>MKKAWCWASYLEEEKAVAVPAKLFKEHQSFPYNKNGFKVGMKLEGVDPEHQSVYCVLTVAEVCGYRIKLHFDGYSDCYDFWVNADALDIHPVGWCEK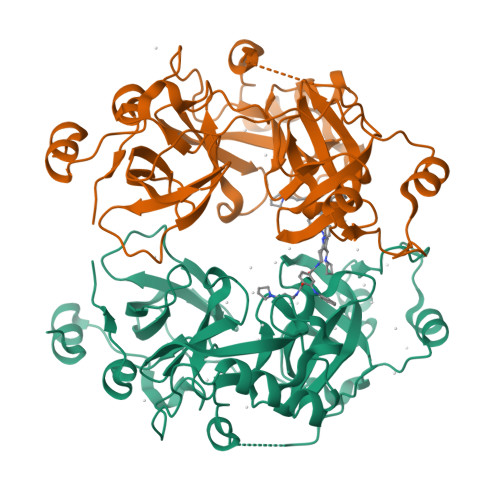TGHKLHPPKGYKEEEFNWQTYLKTCKAQAAPKSLFENQNITVIPSGFRVGMKLEAVDKKNPSFICVATVTDMVDNRFLVHFDNWDESYDYWCEASSPHIHPVGWCKEHRRTLITPPGYPNVKHFSWDKYLEETNSLPAPARAFKVKPPHGFQKKMKLEVVDKRNPMFIRVATVADTDDHRVKVHFDGWNNCYDYWIDADSPDIHPVGWCSKTGHPLQPPLSPLELMEASHHHHHH[2x]> MGSSHHHHHHHHHHSSGLVPRGSHMDGKISILVLGADKAQGGQSRTDSIMVVQYDFINKKMKMMSVMRDIYADIPGYGKHKINSAYALGGPELLRKTLDKNLGINPEYYAVVDFTGFEKMIDELMPEGVPINVEKDMSKNIGVSLKKGNHRLNGKELLGYARFRHDPEGDFGRVRRQQQVMQTLKKEMVNFRTVVKLPKVAGILRGYVNTNIPDSGIFQTGLSFGIRGEKDVKSLTVPIKNSYEDVNTNTDGSALQINK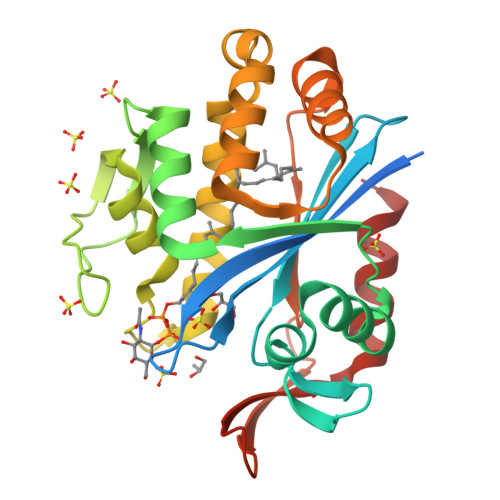NTNKQAIKDFLDED While AMPylases from various pathogenic microorganisms have recently been characterized, the only virulence protein with de-AMPylation activity known to date is the Legionella pneumophila effector SidD which catalyzes AMP removal from the host GTPase Rab1. Here, we present the crystal structure of the de-adenylylation domain of SidD and reveal the catalytic mechanism of Rab1 de-adenylylation. Instead, the catalitic domain of SidD is remarkably similar to that of the metal-dependent protein phosphatases (PPMs), however with distinctive structural features to distinguish AMPylated Rab1 from similarly modified substrates. The finding that SidD is a PPM phosphatase with de-AMPylation activity constitutes a clear example of how L. pneumophila has adapted a common enzymatic fold and mechanism to effectively hydrolyze an unusual substrate.

We identified a proteolytically resistant N-terminal domain (residues 37–350; SidD-NT) that fell within the domain borders of the largest catalytically active domain discovered above and that crystallized readily. The structure of SidD-NT assumed an α/β fold formed by two stacked six-stranded antiparallel β-sheets flanked by α-helices. Pairwise alignment using the DALI server revealed a notable resemblance to metal-dependent protein phosphatases (PPMs), including human PP2Cα and the bacterial PstP which are considered the defining members of this family. In summary, the crystallographic structure of SidD-NT assumes a PPM fold with some conformational rearrangements and the presence of additional subdomains, most of them being grouped around the negatively charged active site. The active site of SidD-NT is located in a negatively charged cleft between the central β-sheets and comprises a relatively well-preserved binuclear metal center. The first metal (M1) is coordinated by four water molecules and residue D110, whereas the second metal (M2) is hexa-coordinated with the classical octahedral geometry formed by four water molecules, D110, and the main chain carbonyl of G111. The M1 position is slightly shifted as compared to other PPMs which can be attributed to the incomplete coordination derived from the absence of a highly conserved aspartic acid residue. Thus, in contrast to other bacterial PPM phosphatases, SidD appears to lack the capacity of binding a third ion at the equivalent M3 position. Quantitative Mg2+ analysis by inductively coupled plasma-optical emission spectrometry (ICP-OES) revealed a stoichiometry of Mg2+ relative to SidD of 1.7 to 1 (data not shown) suggesting that the active site of SidD contains two Mg2+ ions. The structure of the active site revealed the presence of two Mg2+ ions coordinated by D92, D110, D326, the main chain carboxyl of G111, and several water molecules.

> MRSIITQICNGVLHGQSYQSGSNDLDKGNSEIFASSLFVHLNEQGKEIIKHKDSDDKIVIGYTKDGMAFQIVVDGFYGCERQAVFSFIDNYVLPLIDNFSLDLTRYPDSKKVTESLIHTIYSLRSKHAPLAEFTMSLCVTYQKDEQLFCAGFGIGDTGIAIKRNEGTIEQLVCHTEVDGFKDAFDNYSSANIDLVIERNSVFNTKVMPGDELVGYTYVPPMLEMTEKEFEVETVDGKKINKRIVRHLNLDPGNFDDKDPLFSQLLQVVKSKQKQLVEQAKETGQIQRFGDDFTVGRLVIPDQLLINQLRIHALSHHHHH> PVDMSNLFYKTLLDDFSRSLEMQPLVFDDHGTCNMIIDNTFALTLSCDYARERLLLIGLLEPHKDIPQQCLLAGALNPLLNAGPGLGLDEKSG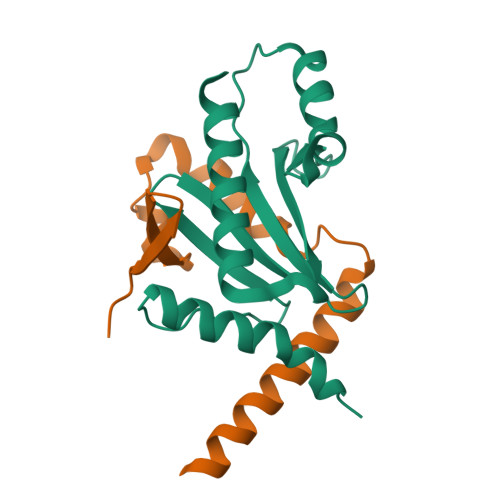LYHAYQSIPREKLSVPTLKREMAGLLEWMRGWREA;> IPALKANGQLEVDGKRYEIRAADDGTISVLRPEQQSKAKSFFKGASQLIGGSSQRAQIAQALNEKVASARTVLHQSAMTGGR> MLPQRLHPSRLLALALFSLVLGLAGCQTKPPQTGLSAEQIAVLQEQGFELRDEGWEFGMS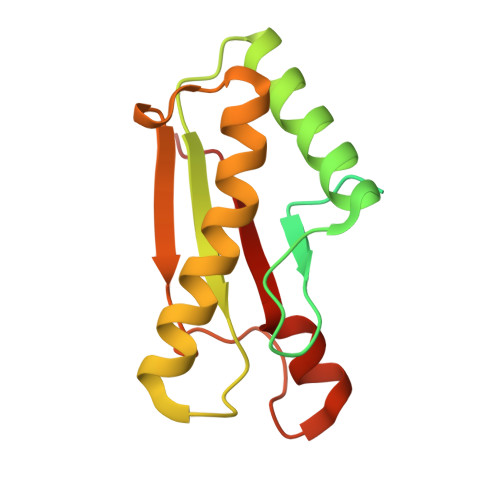SKVLFGNNLDRLNPDSRNTLTKIARALLAVDIDKVRLEGHTDNYGDEGYNQKLSERRAESVAAVFREAGMPAANIEVRGLGMSKPVADNKTRAGRSENRRVAIIVPAE> GAMDPRKGYKVLAIETSCDDTCVSVLDRFSKSAAPNVLANLKDTLDSIDEGGIIPTKAHIHHQARIGPLTERALIESNA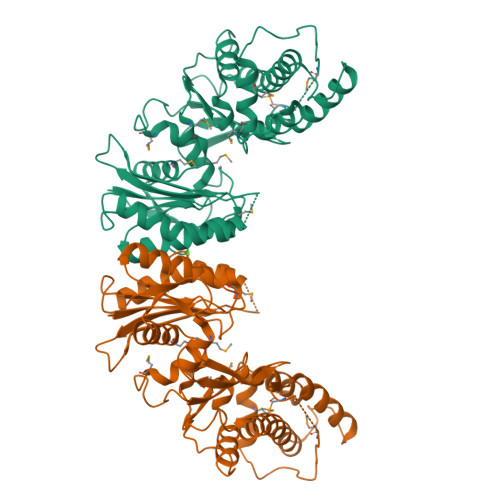REGIDLICVTRGPGMPGSLSGGLDFAKGLAVAWNKPLIGVHHMLGHLLIPRMGTNGKVPQFPFVSLLVSGGHTTFVLSRAIDDHEILCDTIDIAVGDSLDKCGRELGFKGTMIAREMEKFINQDINDQDFALKLEMPSPLKNSASKRNMLSFSFSAFITALRTNLTKLGKTEIQELPEREIRSIAYQVQESVFDHIINKLKHVLKSQPEKFKNVREFVCSGGVSSNQRLRTKLETELGTLNSTSFFNFYYPPMDLCSDNSIMIGWAGIEIWESLRLVSDLDICPIRQWPLNDLLSVDGWRTDQL> PKPVVTAVSSTMPVVGSTVTITGQNFIEVSRVNINGEFDIPVGDITTSNTFDEISFVLPQAPTQSGHISVTAIGGTVESAEIFYPLENVILNYDGIGSHVWGDCSFVVADGSSAPYVSNGTCLGITGTVSASNYWWKQSYSNAQWVNTSIIPGNIPIDDLKLQFECFVKEVFTGPVFQIAMCENFDAALNGYVPVSSFTGKTETGKWM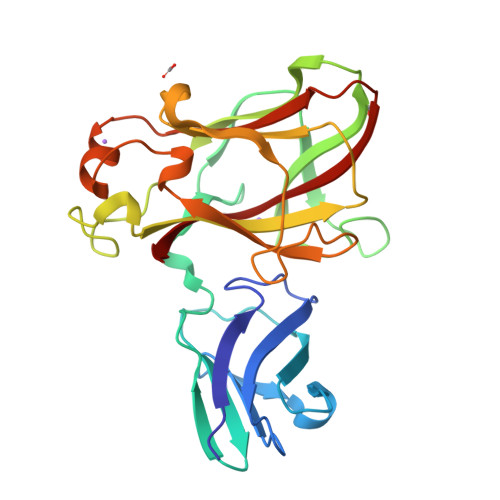QCSVSLSSVVADATYQDFLNRNSTHIGVYATNPGSSQATIEVYFDNFRIVRK> MFKKFDEKENVSNCIQLKTSVIKGIKNQLIEQFPGIEPWLNQIMPKKDPVKIVRCHEHIEILTVNGELLFFRQREGPFYPTLRLLHKYPFILPHQQVDKGAIKFVLSGANIMCPGLTSPGAKLYPAAVDTIVAIMAEGKQHALCVGVMKMSAEDIEKVNKGIGIENIHYLNDGLWHMKTYK;> GDYPLRVLYCGVCSLPTEYCEYMPDVAKCRQWLEKNFPNEFAKL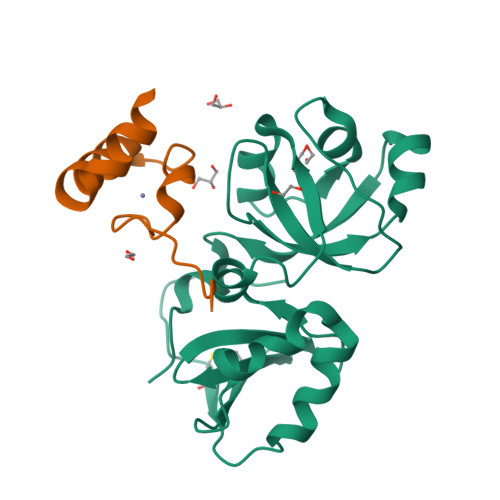TV>MGKVYKKVELVGTSEEGLEAAIQAALARARKTLRHLDWFEVKEIRGTIGEAGVKEYQVVLEVG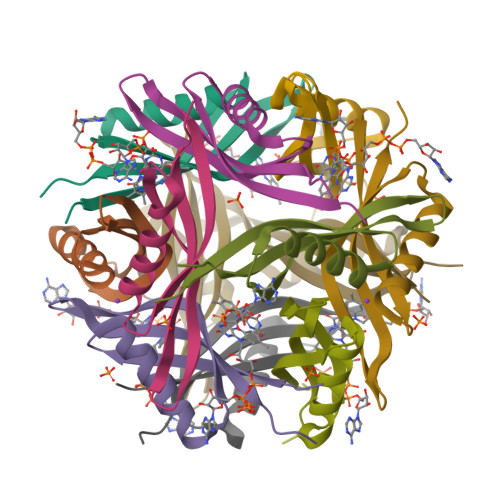FRLEET[8x]>KAIVVQPKDTVDRVAKILSRNKAGSAVVMEGDEILGVVTERDILDKVVAKGKNPKEVKVEEIMTKN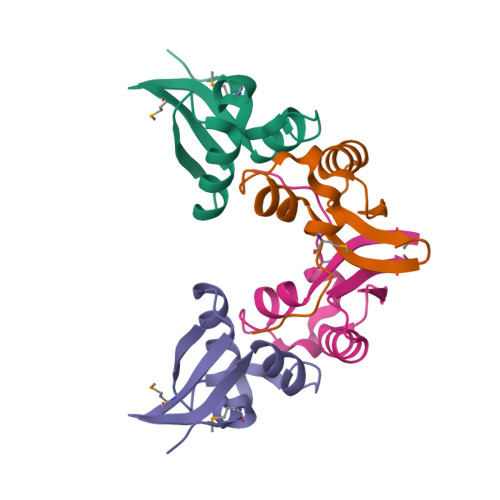PVKI[2x]> MSLARTEKIYIYGASGHGLVCEDVAK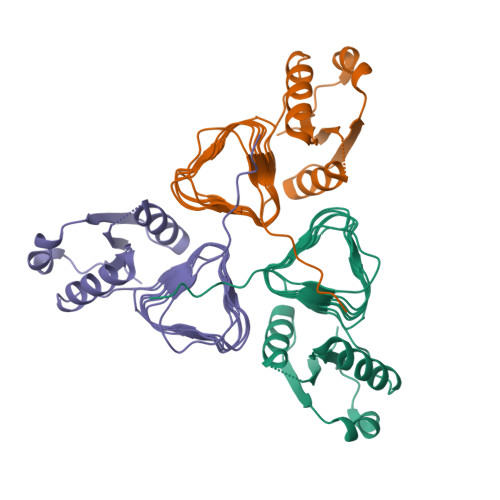NMGYKECIFLDDFKGMKFESTLPKYDFFIAIGNNEIRKKIYQKISENGFKIVNLIHKSALISPSAIVEENAGILIMPYVVINAKAKIEKGVILNTSSVIEHECVIGEFSHVSVGAKCAGNVKIGKNCFLGINSCVLPNLSLADDSILGGGATLVKNQDEKGVFVGVPAKRMEGGSHHHHHH>[2x]MQPVVVIPPDSGKEEEQMASESSKPASQNTETKATIARKGEGSVLEQIDQGSILKLPSNLLFENATSDAINQDMMLYIERIAKIIQKLPKRVHINVRGFTDD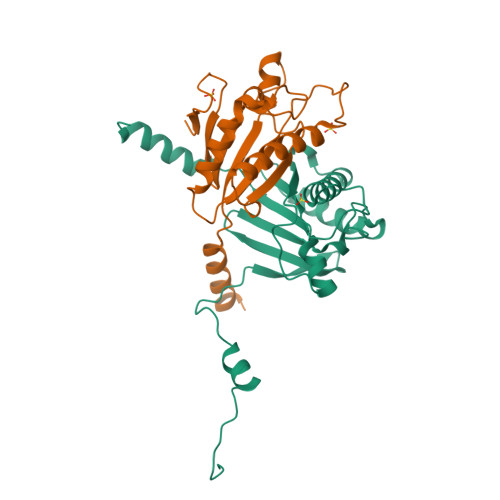TPLVKTRFKSHYELAANRAYRVMKVLIQYGVNPNQLSFSSYGSTNPIAPNDSLENRMKNNRVEIFFSTDANDLSKIHSILDNEFNPHKQQE> GMSDLVFYDVASTGANGFDPDAGYMDFCVKNAESLNLAAVRIFFLNAAKAKAALSRKPERKANPKFGEWQVEVINNHFPGNRNNPIGNNDLTIHRLSGYLARWVLDQYNENDDESQHELIRTTIINPIAESNGVGWDSGPEIY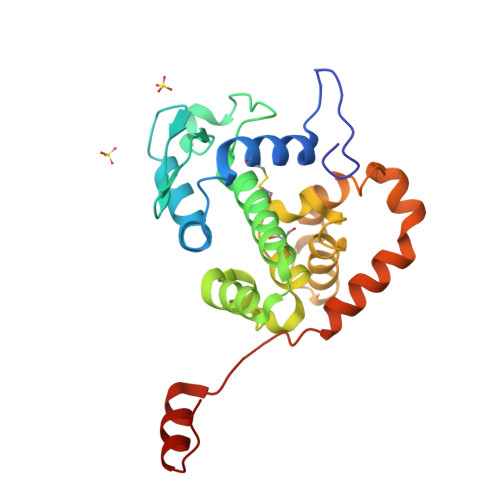LSFFPGTEMFLETFKFYPLTIGIHRVKQGMMDPQYLKKALRQRYGTLTADKWMSQKVAAIAKSLKDVEQLKWGKGGLSDTAKTFLQKFGIRLP2-{4-[4-(4-{4-[2-(2-AMINO-4-OXO-4,7-DIHYDRO-3H-PYRROLO[2,3-D]PYRIMIDIN-5-YL)-ETHYL]-BENZOYLAMINO}-4-CARBOXY-BUTYRYLAMINO)-4-CARBOXY-BUTYRYLAMINO}-PENTANEDIOIC 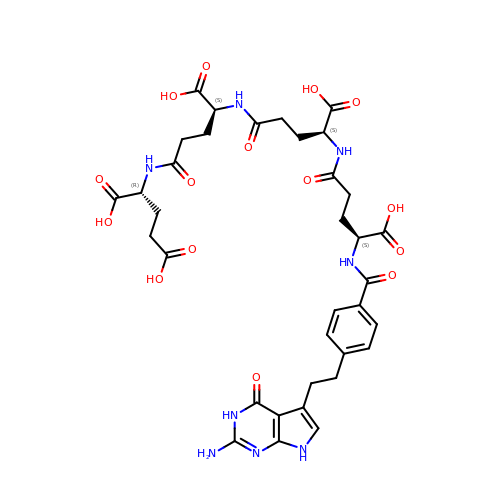ACID | C35 H42 N8 O15 | DICHBVJYDUDAIQ-QEGIFBSNSA-N> GPLGSMASSDVKPKSVSHAKKWSEEIENLYRFQQAGYRDETEYRQVKQVSMVDRWPETGYVKKLQRRDNTFYYYNKQRECDDKEVHKVK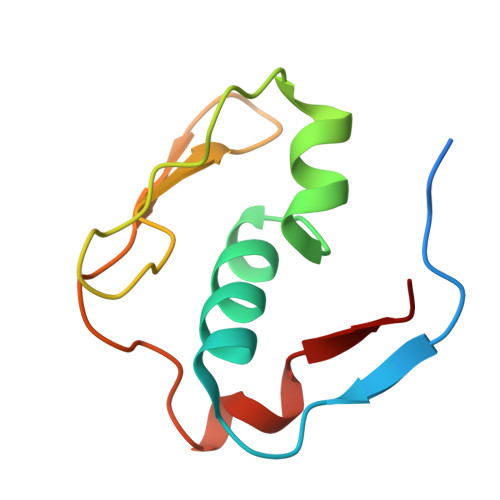IYAY> MVLYFIGLGLYDERDIT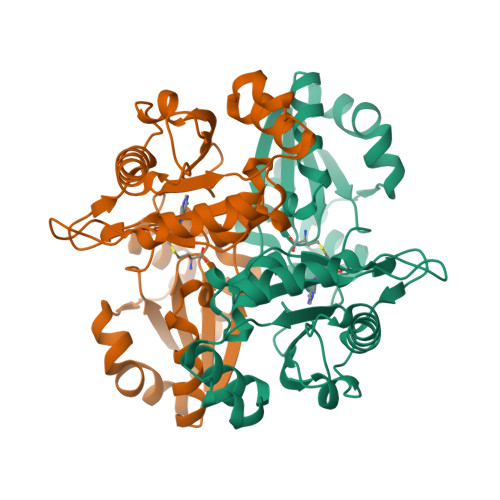VKGLEIAKKCDYVFAEFYTSLMAGTTLGRIQKLIGKEIRVLSREDVELNFENIVLPLAKENDVAFLTPGDPLVATTHAELRIRAKRAGVESYVIHAPSIYSAVGITGLHIYKFGKSATVAYPEGNMFPTSYYDVIKENAERGLHTLLFLDIKAEKRMYMTANEAMELLLKVEDMKKGGVFTDDTLVVVLARAGSLNPTIRAGYVKDLIREDFGDPPHILIVPGKLHIVEAEYLVEIAGAPREILRVNV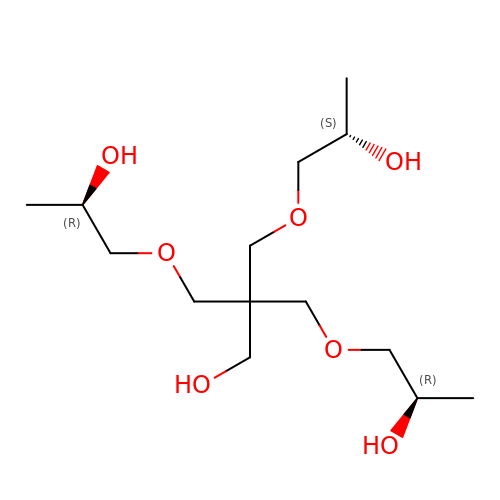3-[(2~{R})-2-oxidanylpropoxy]-2-[[(2~{R})-2-oxidanylpropoxy]methyl]-2-[[(2~{S})-2-oxidanylpropoxy]methyl]propan-1-ol | C14 H30 O7 | KKXXPTIHUVGGLQ-UPJWGTAASA-N> MQLETAELEKGLVRTLVDVIGHRLARDKNNRPNVIRAYPSDNSNDKGLKPDQPFITVYCQDAATPYGWVLD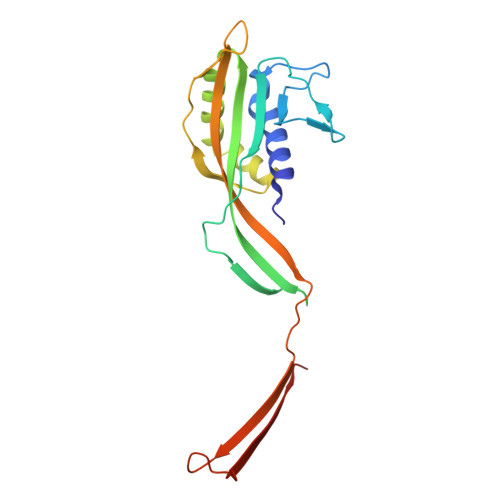KFVEDDVVCYRIAFQIPVLITVNGKGAHSIMLELKQRLEMSSVRDLILEETGATVLDTGAIPNDYTYLNTDFENSAPLVVTLVKNSVLKDERGSIIERVIVDGELVYEEGQEPPEYTIHLDVDSKGVK> ER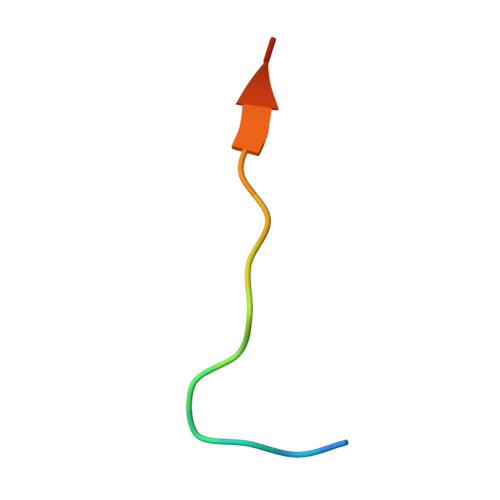MRPFKRQGSVRRRV>MERKQSNAHSTFADINEVEDEAEQELQQQENNNNKRFSGNRGPNRGKQRPFRGFSRQVSLETGFSVLNRESRERDDKKSLPRSGRSFGGFESGGIINGGDGRKTDFSMFRTKSTLSKQKSLLPSIIRERDIENSLRTEDGETKDDSINENVSAGRYFAALRGPELDEVKDNEDILLPKEEQWPFLLRFPIGCFGICLGLSSQAVLWLALAKSPATNFLHITPLINLVVWLFSLVVLVSVSFTYILKCIFYFEAVKREYFHPVRVNFFFAPWVVCMFLAISVPPMFSPNRKYLHPAIWCVFMGPYFFLELKIYGQWLSGGKRRLCKVANPSSHLSVVGNFVGAILASKVGWDEVAKFLWAVGFAHYLVVFVTLYQRLPTSEALPKELHPVYSMFIAAPSAASIAWNTIYGQFDGCSRTCFFIALFLYISLVARINFFTGFKFSVAWWSYTFPMTTASVATIKYAEAVPGYPSRALALTLSFISTAMVCVLFVSTLLHAFVWQTLFPNDLAIAITKRKLTREKKPFKRAYDLKRWTKQALAKKISAEKDFEAEEESHH[3x]

Slow anion channel 1 (SLAC1), an S-type (slow) anion channel of the SLAC/SLAH family which is preferentially expressed in guard cells, has been identified to be mainly responsible for the stress-induced anion efflux and thus playing a pivotal role mediating stomatal closure. Similar to HiTehA and BdSLAC1, AtSLAC1 forms a homotrimer that is tightly packed in the transmembrane domain. Each monomer contains ten transmembrane segments (TMs) that are arranged in two pentagonal layers, with TM1/3/5/7/9 in the inner layer and TM2/4/6/8/10 in the outer layer. Though assembled into a trimeric structure, each subunit of AtSLAC1 functions as an independent anion pore.

We turned to the phosphorylation site mutants which had impaired anion currents and might be stabilized in an inactivated conformation, specifically, the S59A mutant, which has been shown extensively to trim down AtSLAC1 activation and stomatal closure and also has notable reduced currents in the HEK293 cells. In this study, we report the structure of a SLAC1 mutant from Arabidopsis thaliana (AtSLAC1 S59A) in an inactivated state at 2.7 Å resolution as determined by cryo-electron microscopy (cryo-EM) single-particle analysis. In the built atomic model, the N-terminus starts at residue 150, and the C-terminus ends at residue 517. Pore radius analysis of the AtSLAC1 structure reveals that the upper half of the channel is wide open to the periplasmic side of the cell, whereas the lower half is completely sealed. Thus, the AtSLAC1 S59A mutant is in an inactivated, closed state in our determined cryo-EM structure. A large part of the cytosolic domain composed of the N- and C-terminus is clearly identified and forms a plug-like structure which interacts with the transmembrane domain (TMD) and blocks the anion pore, hence inhibiting channel opening. To be noticed, the intracellular surface of the transmembrane domain has a positive electrostatic potential, while the plug has a complementary negative electrostatic potential facing the TMD, suggesting strong electrostatic interactions between the TMD and the plug. E164 in the N-terminus forms a hydrogen bond with Y448 in TM9, and D166 in the N-terminus forms an ionic interaction with R263 in TM3. Besides, R263 also interacts with D507 in the C-terminus. Although the Y448A single mutation retained the activated anion currents, the S59A/Y448A double mutation did not exhibit apparent anion currents. Taken together, breaking the interactions between the intracellular plug and TMs can trigger AtSLAC1 activation even in the absence of the key site phosphorylation, and the cytosolic plug observed in the AtSLAC1 S59A structure, especially the N-terminal tail, may serve as a pore blocker prior to phosphoactivation.>TPDCVTGKVEYTKYNDEDTFTVKVGDKELFTNRANLQSLLLSAQITGMTVTIKTNA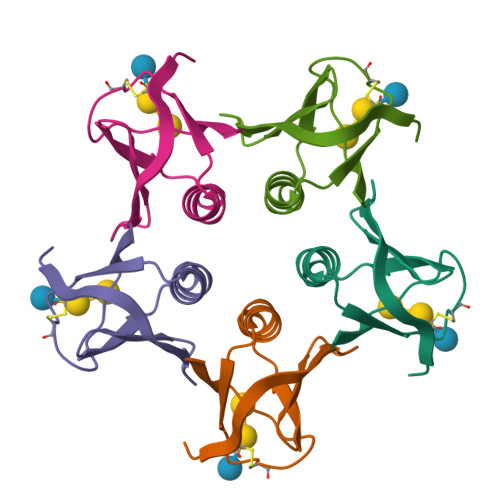CHNGGGFSEVIFR[5x]Kremen 1 and 2 have been identified as co-receptors for Dickkopf (Dkk) proteins, hallmark secreted antagonists of canonical Wnt signaling. Mechanistically it is thought that, in the presence of Dkk, Krm forms a ternary complex with Lrp6, which is then rapidly endocytosed. Structurally, Krm1 and 2 are type I transmembrane proteins with a 40 kDa ectodomain and a flexible cytoplasmic tail consisting of 60–75 residues. KRM1ECD emerges as a rigid molecule with tight interactions stabilizing a triangular arrangement of its Kringle, WSC, and CUB structural domains.

We further succeeded in determination of a low-resolution LRP6PE3PE4-DKK1CRD2-KRM1ECD complex, defining the architecture of the Wnt inhibitory complex that leads to Lrp6 cell-surface depletion. Diffraction data collected from the resulting crystals were highly anisotropic with diffraction extending in the best directions to 3.5 Å and 3.7 Å but only to 6.4 Å in the third direction. Despite the lack of high-resolution diffraction, the general architecture of the ternary complex is revealed. DKK1CRD2 is sandwiched between LRP6PE3 and KRM1Kringle-WSC. KRM1ECD does indeed bind on the opposite side of DKK1CRD2 with only its KR and WSC domains engaged in binding. Although present in the complex subjected to crystallization, we observe no density that could correspond to CRD1 or the domain linker (L). Overall, the DKK1-KRM1 interface is characterized by a large number of polar interactions but only few hydrophobic contacts. The crystal structure gives an explanation for DKK1 loss-of-binding mutations identified previously (Wang et al., 2008): R191 of DKK1 forms a double salt bridge to D125 and E162 of KRM1. Similarly, the K226 side chain of DKK1, which points to a small hydrophobic pocket on the surface of KRM1 formed by Y108, W94, and W106, forms salt bridges with the side chains of KRM1 D88 and D90. The LRP6PE3PE4-DKK1CRD2-KRM1ECD complex structure reveals no direct interactions between KRM1 and LRP6.

> ADPEAFLLFSRRADIRRISLETNNNNVAIPLTGVKEASALDFDVTDNRIYWTDISLKTISRAFMNGSALEHVVEFGLDYPEGMAVDWLGKNLYWADTGTNRIEVSKLDGQHRQVLVWKDLDSPRALALDPAEGFMYWTEWGGKPKIDRAAMDGSERTTLVPNVGRANGLTIDYAKRRLYWTDLDTNLIESSNMLGLNREVIADDLPHPFGLTQYQDYIYWTDWSRRSIERANKTSGQNRTIIQGHLDYVMDILVFHSSRQSGWNECASSNGHCSHLCLAVPVGGFVCGCPAHYSLNADNRTCSAPTTFLLFSQKSAINRMVIDEQQSPDIILPIHSLRNVRAIDYDPLDKQLYWIDSRQNMIRKAQEDGSQGFTVVVSSVPSQNLEIQPYDLSIDIYSRYIYWTCEATNVINVTRLDGRSVGVVLKGEQDRPRAIVVNPEKGYMYFTNLQERSPKIERAALDGTEREVLFFSGLSKPIALALDSRLGKLFWADSDLRRIESSDLSGANRIVLEDSNILQPVGLTVFENWLYWIDKQQQMIEKIDMTGREGRTKVQARIAQLSDIHAVKELNLQEYRQHPCAQDNGGCSHICLVKGDGTTRCSCPMHLVLLQDELSCGEP;> PECFTANGADYRGTQNWTALQGGKPCLFWNETFQHPYNTLKYPNGEGGLGEHNYCRNPDGDVSPWCYVAEHEDGVYWKYCEIPACQMPGNLGCYKDHGNPPPLTGTSKTSNKLTIQTCISFCRSQRFKFAGMESGYACFCGNNPDYWKYGEAASTECNSVCFGDHTQPCGGDGRIILFDTLVGACGGNYSAMSSVVYSPDFPDTYATGRVCYWTIRVPGASHIHFSFPLFDIRDSADMVELLDGYTHRVLARFHGRSRPPLSFNVSLDFVILYFFSDRINQAQGFAVLYQAVK;> KGQEGSVCLRSSDCASGLCCARHFWSKICKPVLKEGQVCTKHRRKGSHGLEIFQRCYCGEGLSCRIQKDHHQASNSSRLHTCQRH> GMPQTITRGIKAMLDEANSSIETLTTADAIALHK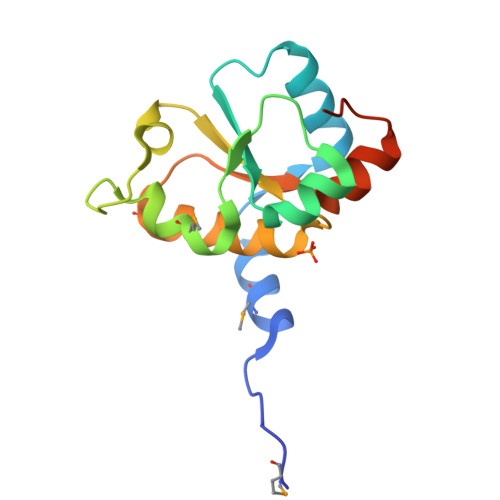SGASDVVIVDIRDPREIERDGKIPGSFSCTRGMLEFWIDPQSPYAKPIFQEDKKFVFYCAGGLRSALAAKTAQDMGLKPVAHIEGGFGAWRDAGGPIEAWAPKKK> AASVYTLPAGADFLMCYSVAEGYYSHRETVNGSWYIQDLCEMLGKYGSSLEF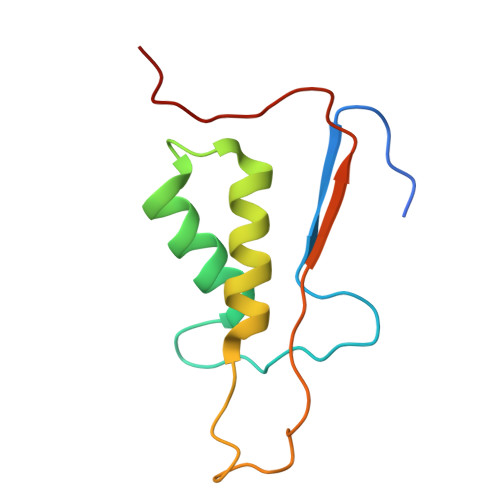TELLTLVNRKVSQRRVDFCKDPSAIGKKQVPCFASMLTKKLHFFPKSN> MTIDQKNTNIDPRFPHHHPRPQSFWEARAKALESLLIEKGHLSSDAIERVIKHYEHELGPMNGAKVVAKAWTDPAFKQRLLEDSETVLRELGYYGLQGEHIRVVENTDTVH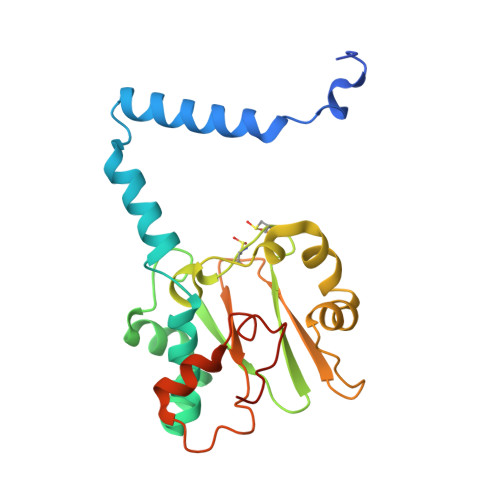NVVVCTLCSCYPWPLLGLPPSWYKEPAYRARVVKEPRQVLKEFGLDLPDSVEIRVWDSSSEIRFMVLPQRPEGTEGMTEEELAKLVTRDSMIGVAKIEPPKVTVG We investigated a TRPM2 chanzyme from choanoflagellates that integrates two seemingly incompatible functions into a single peptide: a channel module activated by ADP-ribose with high open probability and an enzyme module (NUDT9-H domain) consuming ADP-ribose at a remarkably slow rate. Using time-resolved cryogenic-electron microscopy, we captured a complete series of structural snapshots of gating and catalytic cycles, revealing the coupling mechanism between channel gating and enzymatic activity. The slow kinetics of the NUDT9-H enzyme module confers a self-regulatory mechanism: ADPR binding triggers NUDT9-H tetramerization, promoting channel opening, while subsequent hydrolysis reduces local ADPR, inducing channel closure. The structures of srTRPM2 exhibit a characteristic TRPM architecture, from top to bottom, a transmembrane domain (TMD) layer containing the ion-conducting pore, a signal transduction layer consisting of MHR3/4 domain and the C-terminal rib helix, and an ADPR-sensing layer consisting of the N-terminal MHR1/2 domain and the C-terminal NUDT9-H domain.

The tetramerization of the NUDT9-H domain through the buckle helix remodels the interface between the enzymatic module and the channel module. This raises the question of whether the NUDT9-H enzyme module plays a direct role in channel gating of srTRPM2 on ADPR binding. To this end, we generated a truncated construct by removing NUDT9-H, srTRPM2–ΔNUDT9-H. Despite reduced protein expression level at the plasma membrane, the truncation construct still responded to ADPR and Ca2+, generating currents with similar characteristics to the WT. In agreement with the functional data, the overall structure of srTRPM2–ΔNUDT9-H closely resembles the channel module of srTRPM2, but with some minor conformational changes that may have contributed to the subtle differences in gating kinetics. Our result indicates that the NUDT9-H domain is dispensable for the channel activation of srTRPM2, which is consistent with the nvTRPM2 chanzyme, but plays a role in the regulation of the channel activity. Supporting this idea, both the channel module and enzyme module can be expressed and purified separately, and each is functional.

>[4x]MQRARPGELVEVIMFRPTGKARVSNLDESMAMEFTDLRTRAMSSAAMIRQSVAAKTLLIENEDGKGSTRMEVQDFMKRFHMHASEDDKTGSPSTAWGTLRFPTKEATAPYLRLSVNDDPEDALLFVKAMLAQKYGETYDRPSLILSVTGGARNFTLPPRLETAIAKGLRLAAQRTNAWVVTGGTNTGVMKLTGQIMEALSKTQSHFIPPTIGIATYGVIIGGDDMTRGEPPKIGLEYEMHKKDPPKTTPLDDNHNLFLLVDDGSTNKFGKEIKFRAAFENAAGQAFAAPVVTIVVQGGPGTLGTALQAVRQGTPIVVVDGSGLAADVLAYAYNFMHNPLTRFKSYTIDDLRQKVAQTFNPKSSQQLTNLLDSALECVQDPNLVVVYSLQESGIDEFDDCILKAIFSSQGKLGNKLKQAMYFDQLDVAKRALSEASKNGQHNEIAACINDNLMAAMMHNKPHFVELYLGFDAKIYELKPSEEVAKTNITALDELPSFALAIEELYKREAKKPHSHVQRLVSLSNTDVLGRHYRVSTQRGDGTTRRIGRDLANTRAYNVLRMDQIFARLVSKDFSVNRDFTIYDSKYDKVPGIQFRRTAQASHMLFLWAICLDRFRMARHFWLIGDQSIINALVASRILERLSTHRALQGPHLAEERAKMQHNAKKFEELAVGVLGECHGSDSHMASEMLHSKNDMFNKKNAINIAYDAKSLAFLSHPATQSVINADWYGHLKSVTSFWAVLFAFFFPFFVLPFINFSEDHAEQQVEAPRDFFTDAPRSSHSANSTTSGAHRLRRKFAKFYSAPYTRFISDLLSHFVLCVVTSYFVLDKLEDTISAIEWILLVWFVALLLEELRQMIFCDGIAEYISDTWNRLDLIMITLFFVGFFTHASDPSNQDSKVVSKGIHAFLVVVLWLRFMRYYALSKNLGPKLIMMMEMMKDVSTFVFLLLIFLIGYGVAAQSLLSPDEDFSSRTFIGVLFRPYFQIYGELFLDDLNSEANCLGDTPFTECSRETVRMVPFFLAVYILGSNVLLVNLLIAMFNDTYMKVQEAAEDLWRKQNYELCAEYKDRPFLPAPFILLAHVHMLFMRLLRLCGVHTQEHEKIQDDETKRKITTFEELNTDKFLRRWERERQEMLEARVKMTNDNVVQAMGMMDQLLEHMISFRFSLDQQATKIKQEIRDDGLPSTEPTGLVSRTPSQPINRLNSAVAVHGHTAEAA3-(3-acetamidophenyl)benzoic acid | C15 H13 N 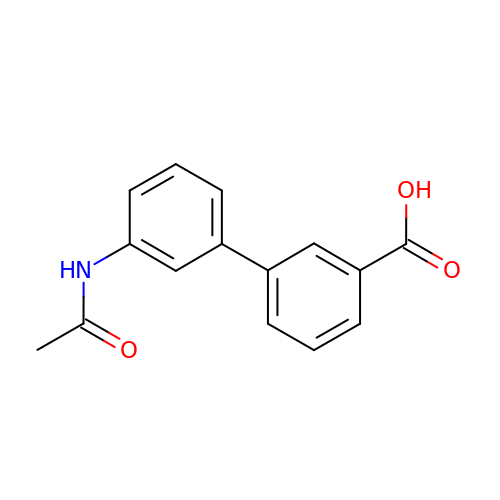O3 | PKQLIAIJVCDASV-UHFFFAOYSA-N>MKLFRVVKRGYYISYAILDNSTIIRLDEDPIKALMRYSENKEVLGDRVTGIDYQSLLKSFQINDIRITKPIDPPEVWGSGISYEMARERYSEE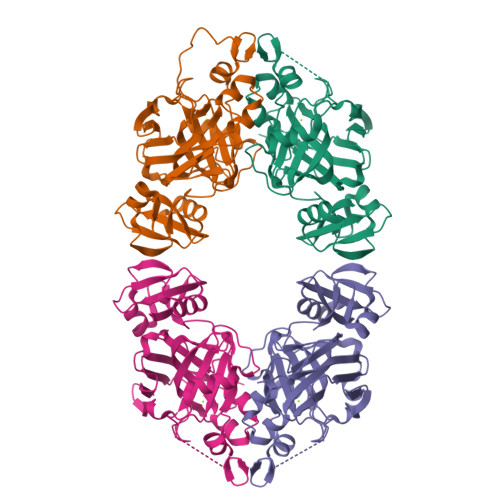NVAKILGKTIYEKVYDAVRPEIFFKATPNRCVGHGEAIAVRSDSEWTLPEPELAVVLDSNGKILGYTIMDDVSARDLEAENPLYLPQSKIYAGCCAFGPVIVTSDEIKNPYSLDITLKIVREGRVFFEGSVNTNKMRRKIEEQIQYLIRDNPIPDGTILTTGTAIVPGRDKGLKDEDIVEITISNIGTLITPVKKRRKIT[4x]> GSHMTSSANEGSHMTSSANEDMPVERILEAELAVEPKTETYVEANMGLNPSSPNDPVTNICQAADKQLFTLVEWA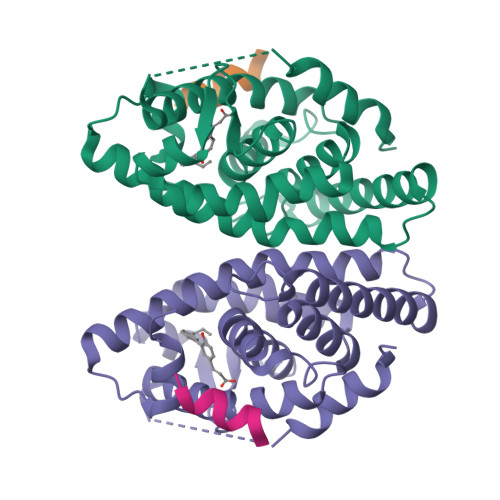KRIPHFSELPLDDQVILLRAGWNELLIASFSHRSIAVKDGILLATGLHVHRNSAHSAGVGAIFDRVLTELVSKMRDMQMDKTELGCLRAIVLFNPDSKGLSNPAEVEALREKVYASLEAYCKHKYPEQPGRFAKLLLRLPALRSIGLKCLEHLFFFKLIGDTPIDTFLMEMLEAPHQMT;> KHKILHRLLQDSS> MSKYSQDVL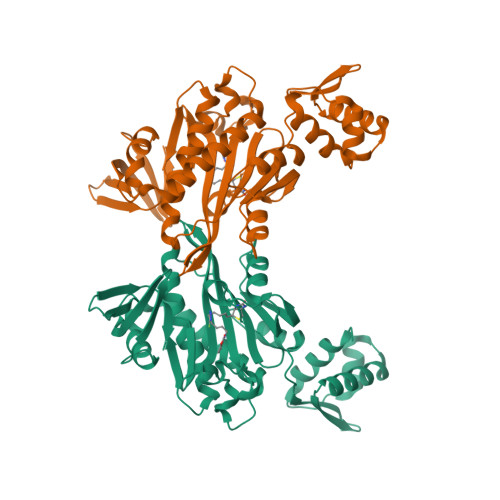QLLYKNKPNYISGQSIAESLNISRTAVKKVIDQLKLEGCKIDSVNHKGHLLQQLPDIWYQGIIDQYTKSSALFDFSEVYDSIDSTQLAAKKSLVGNQSSFFILSDEQTKGRGRFNRHWSSSKGQGLWMSVVLRPNVAFSMISKFNLFIALGIRDAIQHFSQDEVKVKWPNDIYIDNGKVCGFLTEMVANNDGIEAIICGIGINLTQQLENFDESIRHRATSIQLHDKNKLDRYQFLERLLQEIEKRYNQFLTLPFSEIREEYIAASNIWNRTLLFTENDKQFKGQAIDLDYDGYLIVRDEAGESHRLISADIDFHHHHHH> AAPGKPTIAWGNTKFAIVEVDQAATAYNNLVKVKNAADVSVSWNLWNGDTGTTAKVLLNGKEAWSGPSTGSSGTANFKVNKGGRYQMQVALCNADGCTASDATEIVVADTDGSHLAPLKEPLLEKNKPYKQNSGKVVGSYFVEWGVYGRNFTVDKIPAQNLTHLLYGFIPICGGNGINDSLKEIEGSFQALQRSCQGREDFKVSIHDPFAALQKAQKGVTAWDDPYKGNFGQLMALKQAHPDLKILPSIGGWTLSDPFFFMGDKVKRDRFVGSVKEFLQTWKFFDGVDIAWEFPGGKGANPNLGSPQDGETYVLLMKELRAMLDQLSVETGRKYELTSAISAGKDMIDKVAYNVAQNSMDHIFLMSYDFYGAADLKNLGHQTALNAPAWKPDTAYTTVNGVNALLAQGVKPGKIVVGTA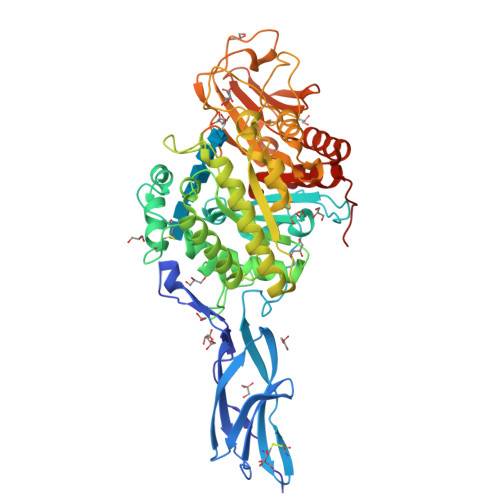MYGRGWTGVNGYQNNIPFTGTATGPVKGTWENGIVDYRQIAGQFMSGEWQYTYDATAEAPYVFKPSTGDLITFDDARSVQAKGKYVLDKQLGGLFSAMIDADNGDILNSMNASLGNSAGVQHHHHHH>[2x]MTKKGDTYNEAWVKDTNGFDILMGQFAHNIENIWGFKEVVIAGPKDY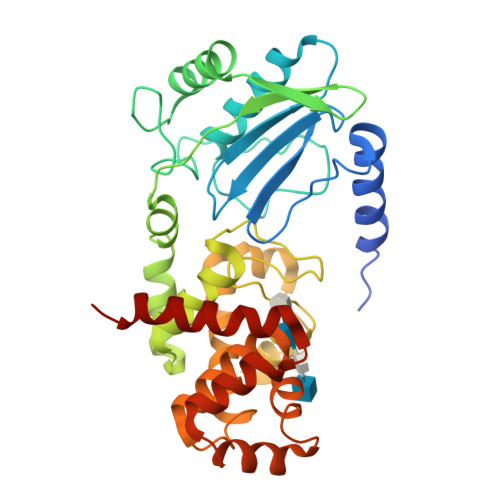VKYTDQYQTRSHINFDDGTITIETIAGTEPAAHLRRAIIKTLLMGDDPSSVDLYSDVDDITISKEPFLYGQVVDNTGQPIRWEGRASNFADYLLKNRLKSRSNGLRIIYSVTINMVPNHLDKRAHKYLGMVRQASRKYGVDESLILAIMQTQSSFNPYAVSRSDALGLMQVVQHTAGKDVFRSQGKSGTPSRSFLFDPASNIDTGTAYLAMLNNVYLGGIDNPTSRRYAVITAYNGGAGSVLRVFSNDKIQAANIINTMTPGDVYQTLTTRHPSAESRRYLYKVNTAQKSYRRR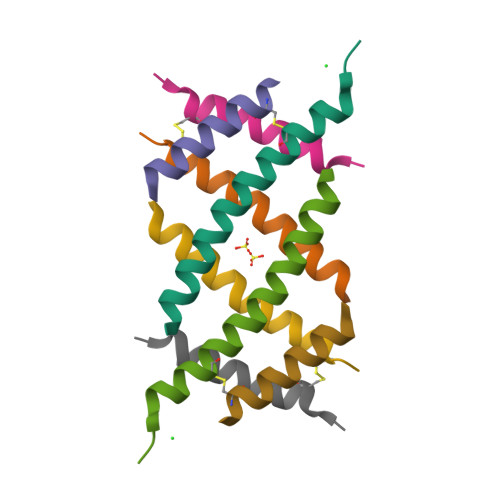>[8x]SEDYERRRSECVSEMLDLEKQFSELKEKLFRERLS> GSHMAATAAEAVASGSGEPREEAGALGPAWDESQLRSYSFPTRPIPRLSQSDPRAEELIENEEPVVLTDTNLVYPALKW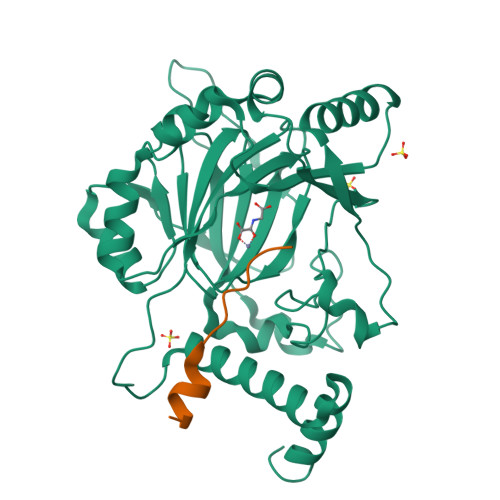DLEYLQENIGNGDFSVYSASTHKFLYYDEKKMANFQNFKPRSNREEMKFHEFVEKLQDIQQRGGEERLYLQQTLNDTVGRKIVMDFLGFNWNWINKQQGKRGWGQLTSNLLLIGMEGNVTPAHYDEQQNFFAQIKGYKRCILFPPDQFECLYPYPVHHPCDRQSQVDFDNPDYERFPNFQNVVGYETVVGPGDVLYIPMYWWHHIESLLNGGITITVNFWYKGAPTPKRIEYPLKAHQKVAIMRNIEKMLGEALGNPQEVGPLLNTMIKGRYN;> HLEVVKLLLEHGADVXAQDK[(2~{R},4~{S})-4-[2-(aminomethyl)imidazol-1-yl]-2-[1-[(4-chlorophenyl)methyl]-5-methyl-indol-2-yl]pyrrolidin-1-yl]-(1~{H}-pyrrolo[2,3-b]pyridin-5-yl)methanone | C32 H30 Cl N7 O | 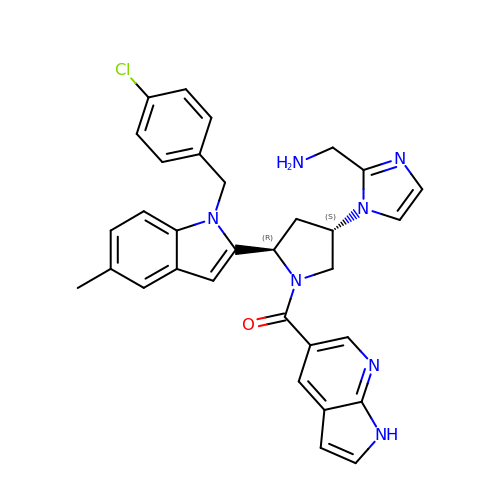IRMSFVCDJOZKRF-LITSAYRRSA-N>MASTVTVDWDTTYQTIDGFGVSEAFHQSNNIARLGETKQNEIYDLLFSTTDGAGFSIFRSILGDGGTWGNADDGPNKTMQPAEDVWDWNESNDDQIPMIRAIQSKYGVDQILYTVWSPPAWMKTNGSVVGGSLRTDKYQAYATYLAEHIKNYKSKFGIEITHIGIQNEPNLETSYSSCRWSPEELRIFMRDYLVPTFDKENITAKVVFAENMSFNEQYAINSLNDPIAVKRVDIVGAHNYGSSYIPFTTTKSKGKGIWMTEVSDMNGNDTTINDGLRWAKEIHDFMTITEGNAWFYWWGACFKTYNGEGLIQMDLNSKTYKVAKRLYTIGQFSRFIRPGWQRIEATKNPV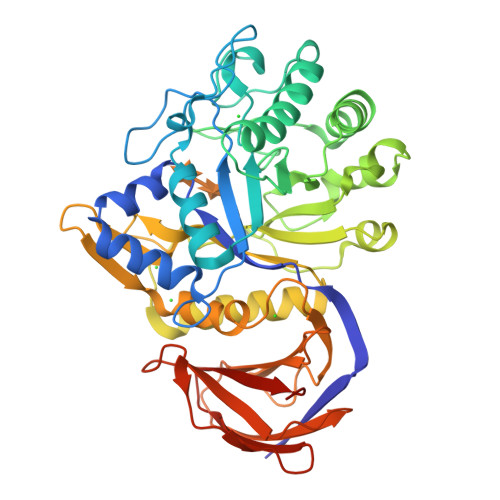SNVYVTAYKDPKTGKFAIVAINNGWSKQSITYTLKGFSPASVTPYTTSSTQNLEKGSDITVNNSSFSFELAPNSITTFVGDTESASLEHHHHHH[2x]> MKKIAVLTSGGDSPGMNAAVRAVVRTAIYNEIEVYGVYHGYQGLLNDDIHKLELGSVGDTIQRGGTFLYSARCPEFKEQEVRKVAIENLRKRGIEGLVVIGGDGSYRGAQRISEECKEIQTIGIPGTIDNDINGTDFTIGFDTALNTIIGLVDKIRDTASSHARTFIIEAMGRDCGDLALW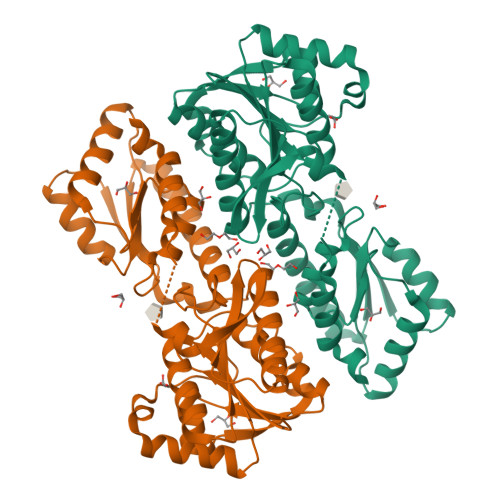AGLSVGAETIVVPEVKTDIKEIADKIEQGIKRGKKHSIVLVAEGCMTAQDCQKELSQYINVDNRVSVLGHVQRGGSPTGADRVLASRLGGYAVDLLMQGETAKGVGIKNNKIVATSFDEIFDGKDHKFDYSLYELANKLSILEHHHHHH>MALSTATKAATDALAANRAPTSVNAQEVHRWLQSFNWDFKNNRTKYATKYKMANETKEQFKLIAKEYARMEAVKDERQFGSLQDAL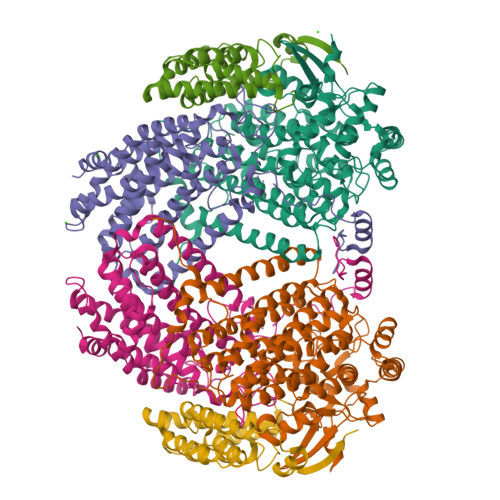TRLNAGVRVHPKWNETMKVVSNFLEVGEYNAIAATGMLWDSAQAAEQKNGYLAQVLDEIRHTHQCAYVNYYFAKNGQDPAGHNDARRTRTIGPLWKGMKRVFSDGFISGDAVECSLNLQLVGEACFTNPLIVAVTEWAAANGDEITPTVFLSIETDELRHMANGYQTVVSIANDPASAKYLNTDLNNAFWTQQKYFTPVLGMLFEYGSKFKVEPWVKTWDRWVYEDWGGIWIGRLGKYGVESPRSLKDAKQDAYWAHHDLYLLAYALWPTGFFRLALPDQEEMEWFEANYPGWYDHYGKIYEEWRARGCEDPSSGFIPLMWFIENNHPIYIDRVSQVPFCPSLAKGASTLRVHEYNGEMHTFSDQWGERMWLAEPERYECQNIFEQYEGRELSEVIAELHGLRSDGKTLIAQPHVRGDKLWTLDDIKRLNCVFKNPVKAFN[2x];>SMLGERRRGLTDPEMAEVILKALPEAPLDGNNKMGYFVTPRWKRLTEYEALTVYAQPNADWIAGGLDWGDWTQKFHGGRPSWGNETTELRTVDWFKHRDPLRRWHAPYVKDKAEEWRYTDRFLQGYSADGQIRAMNPTWRDEFINRYWGAFLFNEYGLFNAHSQGAREALSDVTRVSLAFWGFDKIDIAQMIQLERGFLAKIVPGFDESTAVPKAEWTNGEVYKSARLAVEGLWQEVFDWNESAFSVHAVYDALFGQFVRREFFQRLAPRFGDNLTPFFINQAQTYFQIAKQGVQDLYYNCLGDDPEFSDYNRTVMRNWTGKWLEPTIAALRDFMGLFAKLPAGTTDKEEITASLYRVVDDWIEDYASRIDFKADRDQIVKAVLAGLK[2x];>[2x]AKLGIHSNDTRDAWVNKIAQLNTLEKAAEMLKQFRMDHTTPFRNSYELDNDYLWIEAKLEEKVAVLKARAFNEVDFRHKTAFGEDAKSVLDGTVAKMNAAKDKWEAEKIHIGFRQAYKPPIMPVNYFLDGERQLGTRLMELRNLNYYDTPLEELRKQRGVRVVHLQSPH N-[(R)-hydroxy(methyl)phosphoryl]-D-glutamic 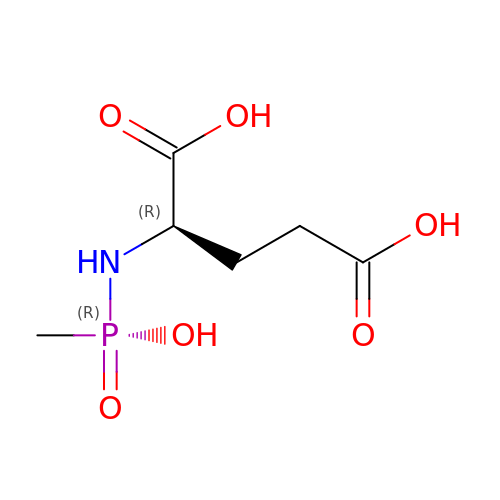acid | C6 H12 N O6 P | XVXVUGZUKCQIOK-SCSAIBSYSA-N>[2x]MKTSSFRNTYAQISLQALKENAASFKASLQSPACRLMAVVKGDGYGHGAVAAASSALNGGADYLGVAILDEAIELRDAGVEAPILVLGYTSPHALREAISRNITLTVFSTDVRDALLEVASEAESPIKVHIKTETGMGRVGVQTKEELLDVMTPLYHHNNIEVEGIFTHFAEADNLQSTYTDEQFARFLSFIEAIEKDDMHVPIKHCCNSAG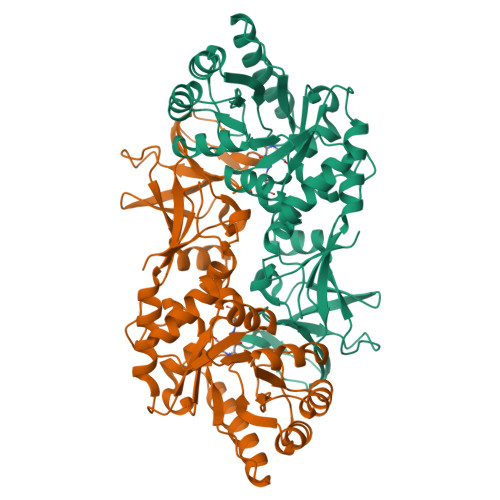TLFHKDKHLDMVRVGISLYGLRPDVSLEFPIELTQAMRLFSSIVSLRKLPEGSSISYGRTHKLSSEKVVATMPIGYADGLSRALSNKGFVTLHGQKAPILGRVCMDQTMIDVTDIPDAALGDHVEFPIDEMAELTGTINYEIVCAVSKRVPRYYEEN> MASSASKFSKIVVGNETHKSARNVLEGFAKDIKGKASIDAEKHAYSLKGNLKDAKFNHDFFKIKSDMPGNPCYLDFAFHSNTPGNQREYRHPCARSMNKNLFNLEGAVCTNSKIKGNEEKINGAGACAPYRRRHICDLNLEHIDVHNVQNIHDLLGNVLVTAKYEGESIVEKHPNRGSSEVCTALARSFADIGDIIRGKDLYLGHEQGNNKLEARLKTIFQNIKNKNKSPLDKLSLEQVREYWWALNREDVWKALTCFADGSEEYFIQSSDKEHSFSSEYCGHEQGNVPTNLDYVPQFLRWFDEWADDFCRIKKIKLENVKNACRDEKKRKYCSLNGFDCTQTIWKKGVLHRSNECTGCLVKCNPYEIWLGNQREAFRKQKEKYENEIKTYVHDTGISNSNINNEYYKEFYKILKNNNYETANEFIKLLNEGRYCNKKEKIEEEEDIDFTNTNEKGTFYRSDYCQVCPDCGVECKNETCTPKTVIYPDCGKNEKYEPPGDAKNTEINVINSGDKEGYIFEKLSEFCTNENNENGKNYEQWKCYYDNKKNNNKCKMEINIANSKLKNKITSFDEFFDFWVRKLLIDTIKWETELTYCIN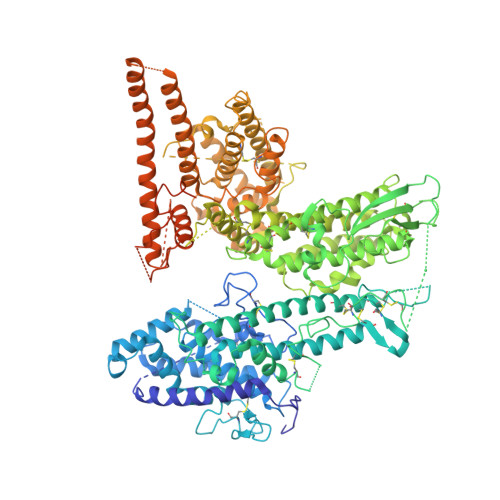NTDVTDCNKCNKNCVCFDKWVKQKEDEWTNIMKLFTNKHDIPKKYYLNINDLFDSFFFQVIYKFNEGEAKWNELKENLKKQIASSKANNGTKDSEAAIKVLFNHIKEIATICKDNNTNEGCDPSVDSKTNSCGKNTKAGSDKVISVKQIAQYYKRIAHKQLNERGSRSALKGDASKGTYKKNGTPSNLKEICEITAKHSNDSRRDGEPCTGKDGGQVRVRTKIGTPWTKIVEINKTSYKEVFLPPRRQHMCTSNLEHLNTGNKGLKDGKLAIHSLLGDVLLAAKEQANFIKNKYKRQKASNGFKDKGTICRAIRYSYADLGDIIKGTDLWEANPGEKNTQRRLKTVFGIIKKNMPGIKDNQKYKDDEKNNPPYKLLREDWWEANRDQVWQAMKCAMKNGITCGSSDHTPLDDYIPQKLRWLTEWAEWYCKAQSKEYEKLKEKCKECKGNDQCTQDTPDCEKCKAACKKYGKNIKTWEDQWKVISSKYKELYKQAEIYAGNGGPGYYNTKVQEEDKPVVDFLYNLYLQNGGKKGPPPDTHPSKSVTAPLKQVATVDTPSTVYSTPEGYIHQEAAMDCKQQHVFCDDNSGGKDDNKQYAFRHQPHDYDEALRCDQRDKPPPESKKVEKAKKEKDENDDGGSHHHHHHGGGSAHIVMVDAYKPTK>[2x]GCGUACGAAGGAGAGGAGAGGAAGAGGAGAGUACGC;>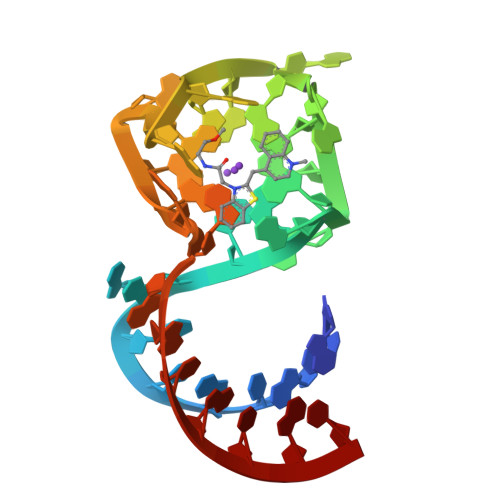 GUACGAAGGAGAGGAGAGGAAGAGGAGAGUAC>[4x]GGSGSGSTALGTLDFSLLYDQENNALHCTISKAKGLKPMDHNGLADPYVKLHLLPGASKANKLRTKTLRNTLNPSWNETLTYYGITDEDMIRK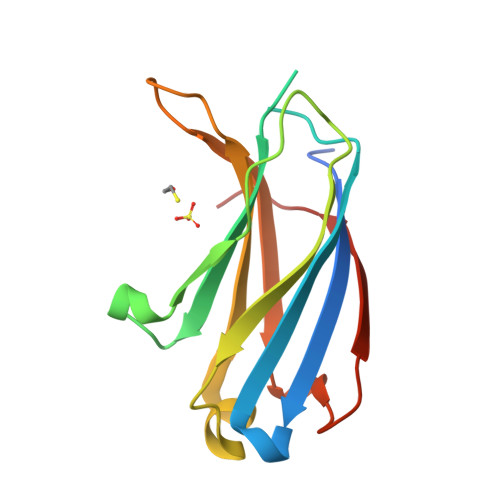TLRISVCDEDKFRHNEFIGETRVPLKKLKPNHTKTFSICLEKQLP> MASRGGTLWHLKEVVIQYSASGNSSQGLRFFFRHLLHRWKQRNPQVQVHTVENKYEAPKATFKYLGERTDSRCETPLKDLSPGQIEQI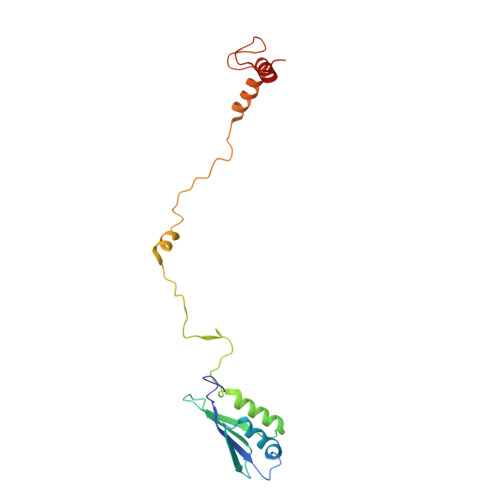LDLHRNSKGDNRFLKHGGPRTWTERRSIQGLWRPSLPSQLIALKWFRRKRPPMRLPKYSPLSLSLSIQAIRGHGRWGSEREFPRGWDQLHLKDILGSPLRSE>[2x]ASMTIVDCGPPDDLPSGRVEYITGPGVTTYKAVIQYSCEETFYTMKVNDGKYVCEADGFWTSSKGEKSLPVCEPVCGLSARTTGGRIYGGQKAKPGDFPWQVLILGGTTAAGALLYDNWVLTAAHAVYEQKHDASALDIRMGTLKRLSPH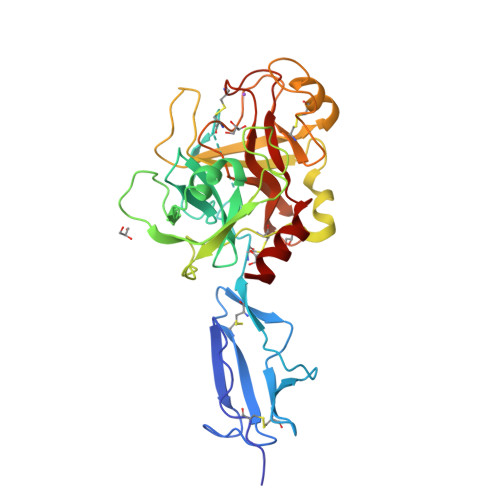YTQAWSEAVFIHEGYTHDAGFDNDIALIKLNNKVVINSNITPICLPRKEAESFMRTDDIGTASGWGLTQRGFLARNLMYVDIPIVDHQKCTAAYEKPPYPRGSVTANMLCAGLESGGKDSCRGDSGGALVFLDSETERWFVGGIVSWGSMNCGEAGQYGVYTKVINYIPWIENIISDF The bifunctional enzyme Δ1-pyrroline-5-carboxylate synthase (P5CS) is vital to the synthesis of proline and ornithine, playing an essential role in human health and agriculture. The P5CS molecule contains two domains, GK and GPR, catalyzing the first and second steps in the biosynthesis of proline from glutamate. The GK domain catalyzes glutamate phosphorylation, and the GPR domain catalyzes the NADPH-dependent reduction of γ-glutamyl phosphate (G5P) to glutamate-γ-semialdehyde (GSA). Our results describe the assembly mechanism of P5CS filaments, in which the GK domain forms tetramer and the GPR domain forms dimer structure, and both domains form specific interaction interfaces.

Filaments in three conditions with (1) glutamate (P5CSGlu), (2) glutamate and ATPγS (P5CSGlu/ATPγS), and (3) glutamate, ATP, and NADPH (P5CSMix) were imaged in cryo-EM for single-particle analysis (SPA). Long and flexible filaments of P5CS were observed under all the three conditions. After 3D classification and 3D reconstruction, the electron density maps of the P5CSGlu, P5CSGlu/ATPγS, and P5CSMix filaments reached resolutions of 4.0 Å, 4.2 Å, and 3.6 Å, respectively (Figure 1—figure supplements 2–4). (C) When all substrates (MgSO4, ATP, NADPH, and glutamate) were added to induce the reaction, the long P5CSMix filaments were observed, which is similar to the P5CSGlu filaments. We chose the P5CSMix filament to display the details. In the helical P5CS filament structure, the GK tetramers serve as the core of the filament, and the GPR dimers form left-handed double helix structures around the central axis. The overall diameter of P5CS filaments in all three states is 180 Å, while the helical twist is 68° and the helical rise is 60 Å. In P5CSGlu/ATPγS and P5CSMix filaments, the additional interface between hook structures pairs locks adjacent GK tetramers. The hook interaction forms strong contacts via hydrogen bonds (M119-R124, L121-M123) and salt bridges (E116-R124). In the P5CSGlu filament, the GK and GPR domains are likely in a stable conformational state, while vibration may occur in the GPR domain of P5CSGlu/ATPγS and P5CSMix filaments due to the binding of ligands. We propose that the interactions among the hook pairs are required for stabilizing the filament during the transformation from the P5CSGlu filament to the P5CSGlu/ ATPγS filament or P5CSMix filament.

>MLQNSFKLAQSLRNGFYRNAWRAFSSHGPRQPLVSPERRLEKAHPTFTERSQLKYARRLVVKLGSAVITREDNHGLALGRLASIVEQVAECHLEGREVMMVTSGAVAFGKQKLAQELLMSLSMRETLNPKDSKEFDGATLEPRAAAAVGQSGLMSLYDAMFAQYGVKIAQVLVTKPDFYNEETRNNLFCTLSELISLNIVPIINTNDAVSPPMFIRDDEPAGGARRGIPIKDNDSLSAMLAAEVQADLLILMSDVDGIYNKPPWEDGAKLMHTYTSDDSNSIEFGKKSKVGTGGMDSKVKAATWALDRGVSVVICNGMQEKAIKTIIGGRKVGTFFTEATESANAVPVEVMAENARTGSRQMQALTPAQRASAVNTLADLLVSREKFILDANAKDLAEAQKSGLAKPLLSRLSLNPAKLKNLSVGLKQIAEDSHKNVGRVLRRTRLADQLELKQVTVPIGVLLVIFESRPDSLPQVAALAMASANGLLLKGGKEAAHSNKALMELVKEALATVGAEHAVSLVSTREEISDLLSMENHIDLIIPRGSSDLVRSIQQQSLHIPVLGHAEGVCHVYIDRDADLEKALRIARDAKCDYPAACNAMETLLIHEDLMSGAIFGDVCNMLKREGVKIYAGPRLNQQLTFGPPAAKSLKHEYGALECCIEVVPSLDEAINHIHTYGSSHTDVIVTENDAAARQFLGSVDSACVFHNASSRFADGFRFGLGAEVGISTARIHARGPVGVEGLLTTKWILEGQDHAAADFAEGGGRTWLHETLPLD[4x]> MQQSL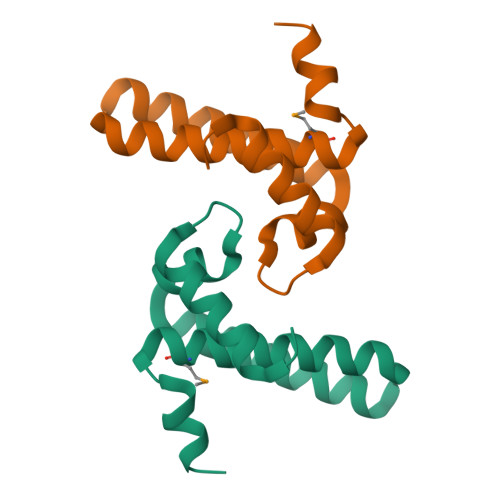AVKTFEDLFAELGDRARTRPADSTTVAALDGGVHALGKKLLEEAGEVWLAAEHESNDALAEEISQLLYWTQVLMISRGLSLDDVYRKL>MIELSLAEALFLILFTGVISMLISRRTGISYVPIFILTGLVIGPLLKLIPRDLAHEIFDFVRVFGLVIILFTEGHNLSWRLLKKNMPTIVTLDTIGLILTALIAGFIFKVVFNSSFLLGFLFGAIIGATDPATLIPLFRQYRVKQDIETVIVTESIFNDPLGIVLTLIAISMLVPGYGGGIFSTLSEKLGIYAGGVIYFLYNVSVSISLGIFLGILGYKFIKRTGIFDFPEIEAFSLSLAFLGFFIGERLDASGYLVATV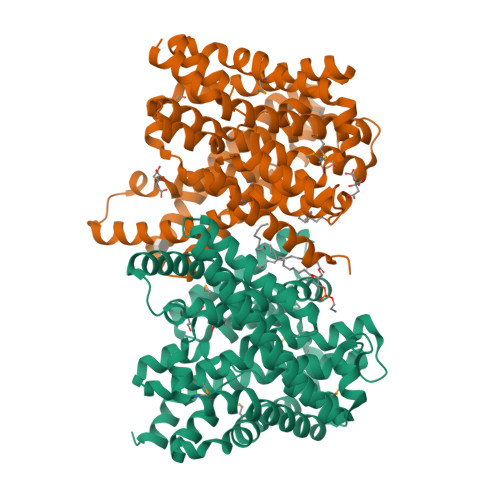TGIVLGNYKLLKPRENIRILKRLQRAIEKEVHFNDTLAALATIFIFVLLGAEMNLEVIWSNLGKGLLVALGVMILARPLATLPLLKWWNFREYLFIALEGPRGVVPSALASLPLSLALKYKSPLLTVHWGEIIMATVVITVLTSVIVETLWIPILKDKLDVG[2x]> XPAPFA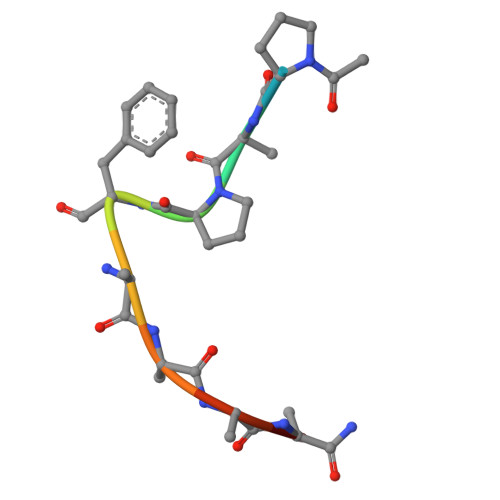AAAX The disease arises in mice and humans from the misfolding of the acute phase protein serum amyloid A1 (SAA1). To investigate the molecular basis of the systemic AA amyloidosis, we here use electron cryo-microscopy (cryo-EM) and determined the structures of AA amyloid fibrils from a patient and from a diseased mouse. The human fibril encloses a clearly discernible cavity that contains many charged and polar amino acid residues, making it likely that the vacant space in the cavity is filled with water. Both fibril proteins adopt all-beta folds and differ sharply from the known globular conformations of SAA family members. The murine and the human fibril possess in-register, parallel cross-β sheets and adopt highly similar β-arch conformations at the protein N-termini.

Corresponding to previous observations, mass spectrometry (MS) shows that the mouse fibril proteins are N-terminal fragments of murine mSAA1.1 protein with mSAA1.1(1–76), mSAA1.1(1–82), and mSAA1.1(1–83) being particularly abundant. The ordered part of the density of the mouse fibril corresponds to residues 1–69 of mSAA1.1, the ordered part of the human fibril to hSAA1.1 residues 2–55. The dominant morphology of the mouse shows a width of 11.8 ± 0.5 nm and a cross-over distance of 75.7 ± 1.3 nm. Platinum side shadowing and TEM demonstrate the left-hand twist of the mouse fibril and its underlying cross-β sheets. The fold of the murine protein is compact and shows a high degree of complementarity. In the murine fibril they wrap around the N-terminal β-arch such that the resulting protein fold superficially resembles the Greek key topology, similar to α-synuclein fibrils. Another substantial difference between the human and the murine fibril protein concerns the packing interface between the two protein stacks. This interface is extremely small in the murine fibril. Two residues (Asp59 and Arg61) make bidentate, reciprocal salt bridges with the respective residues in the opposing protein stack. Each human fibril protein interacts with ten other protein molecules. The non-planarity of the murine fibril protein originates from the tilt of the protein stacks with respect to the fibril axis and a GPGG motif (residues 47–50) that induces a ~5.5 Å height change of the polypeptide chain relative to the fibril axis.

>GFFSFIGEAFQGAGDMWRAYTDMKEAGWKDGDKYFHARGNYDAAQRGPGGVWAAEKISDARESFQEFFGRGHEDTMADQEANR[12x]>[10x]GGGHMGLEKLTWVSEKKPDWSNVQ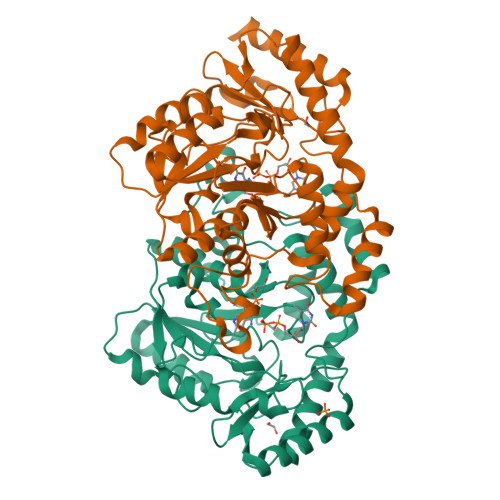KLIAACEATNQYTNIGPIISQLESFIRDSFLIEESKAVIVTSNGTSALHALVGGINRQLGRELKFVTQSFTFPSSNQGPLKDSIIVDIDEDGGLDLNAVKNIEYDGIIVTNIHGNVVDINKYVDFCMNHNKLLIFDNAATGYTFYLGKNSCNYGHASIISFHHTKPFGFGEGGCIIVDRLYENNIRIGLNFGLDNSLGEKSQYSNQASNYRMCDLNAAFILSYLQNNYKKIINRHSEIYEIYKNNLPKRFKLFPNHSKKNPVCSSICLLFDKPFRLDKIPFLSRKYYKPLDLSSPVSLDFYQRILCIPCNIDLTDRQIYEIIGVLNEFADKN>[2x]SNAMSIEKVPILGKETIHVGYGIADHIVREVIANLASSTYVIVTDTNMARTPQYSKLTDDFKTNLSEKRPESRLLTYCVSPGENNKNRATKAAVEDFLLQQGCTRDTVILAVGGGVIGDMIGFVAATFMRGVRVVQVPTTLLAMVD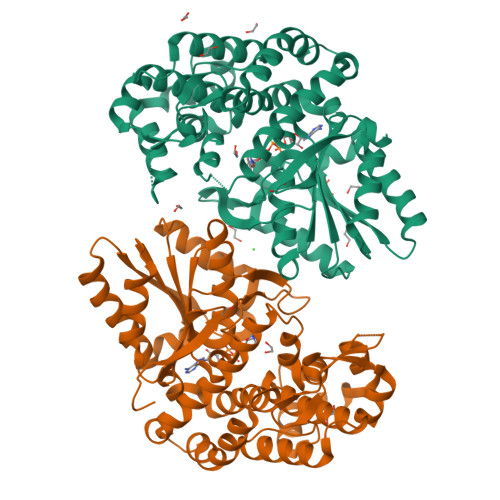SSVGGKTAIDTPLGKNFIGAFHQPEYVFCDVSFLETLPARQFINGMAEVVKTAAIWNEEEFTRLENFSKKFLSVVTSKKPDLQSIKAELVKTVLESVRVKAGVVSSDEKEAGLRNLLNFGHTIGHAIEAVLTPEALHGECVSIGMIKEAELSRYLGILPPVAVARLSKCLVAYGLPVSIDDKEFLKKVGPKRHYVEIDILLKKMAIDKKNDGSKIRCVLLEKIGKCYQLKAHQVSKQDLSFVLT> GRGYEIPARLRTLHNLVIQYASQGRYEVAVPLCKQALEDLEKTSGHDHPDVATMLNILALVYRDQNKYKDAAHLLNDALAIREKTLGKDHPAVAATLNNLAVLYGKRGKYKEAEPLCKRALEIREKVLGKFHPDVAKQLSNLALLCQNQGKAEEVEYYYRRALEIYATRLGPDDPNVAKTK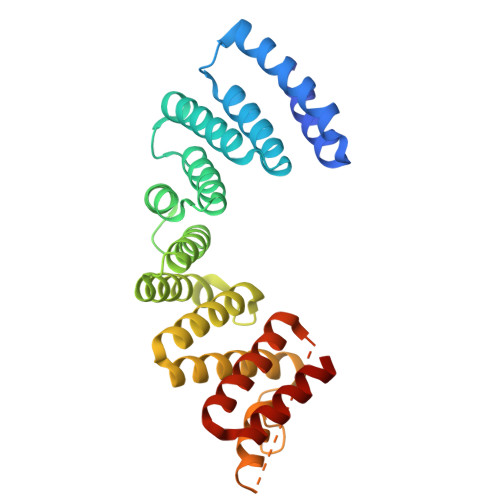NNLASCYLKQGKYQDAETLYKEILTRAHEKEFGSVNGENKPIWMHAEEREESKDKRRDSAPYGEYGSWYKACKVDSPTVNTTLRSLGALYRRQGKLEAAHTLEDCASRSRKR The DNA replication process is a desirable target for an antifungal product; hence, A. fumigatus proliferating cell nuclear antigen (afumPCNA) has been hypothesised as a fungal target for the development of new antifungals. The PCNA processivity factor is also known as the sliding clamp, as DNA slides through its central cavity. PCNA functions as a docking platform to allow DNA polymerases and a host of DNA replication and repair machinery to interact at the replication fork. The PCNA homotrimer comprises two domains, with each containing two alpha helices and nine beta strands, connected by a motif known as the interdomain connecting loop (IDCL), which forms part of the PCNA surface with which binding domain proteins interact.

The co-crystal structure of afumPCNA bound with the p21µ-afumRFC peptide was solved at a resolution of 2.30 Å in order to examine the structural features of an Afum-derived PIP-box. The KRRMP amino acids of the p21µ-afumRFC peptide fold over the PIP-box, not interacting with the afumPCNA’s surface. This is caused by a change in the sequence of the PIP-box compared to the human RFC sequence; the inclusion of a proline residue causes a kink, and the backbone carbonyl of ProXXX interacts with the Asp147 backbone amide and Asn150 residue side chain to stabilize the turn in the peptide. The second arginine, Arg143, is located close to the third arginine, Arg149, producing a loop structure (143–149). The Met144 side chain does not interact with the afumPCNA surface pocket as Gln144 in the p21µ PIP-box does with hPCNA. The Met144 backbone amide does interact with the Asn150 side chain and in turn also interacts with the Asp147 side chain, supporting the 310 helix via extra contacts that hold the compact structure. The p21µ-afumRFC PIP-box has an affinity for afumPCNA of less than 100 nM. This may be accounted for solely by the IIe147, Phe150, and Tyr151 residues, as previous research has shown these conserved residues to be highly favourable, especially IIe147. The two Arg residues can be replaced to create a linkage that, based on the X-ray crystallography structure, would not interrupt the 310-helical conformation and side chain exposure required for binding to afumPCNA, as these are 3.5 Å distance apart in the naturally forming architecture.

>[3x]MLEARLEQASLLKRVVDAIKDLVQDCNFDCNDSGIALQAMDNSHVALVSMLLKAEGFSPYRCDRNIALGINLVSLTKVLRAAQNEDILTLKADDSPDAVNLMFESAETDRISEYDIKLMDIDQEHLAIPETEYAATVEMPSAEFQRICRDLNALSESVVIEATKEGVKFSCQGDIGSGSVTIRQHTSVDKPEQNVSIALSEPVALTFSLKYLVNFCKATSLSSKVTLCLSQEVPLLVEYGLGSGHLRFYLAPKIGDE;>KRRMPTDIRNFFHSKR[3x]N-(3-biphenyl-4-ylpropanoyl)-L-alpha-glutamyl-L-alpha-glutamyl-amide | C25 H29 N3 O7 | 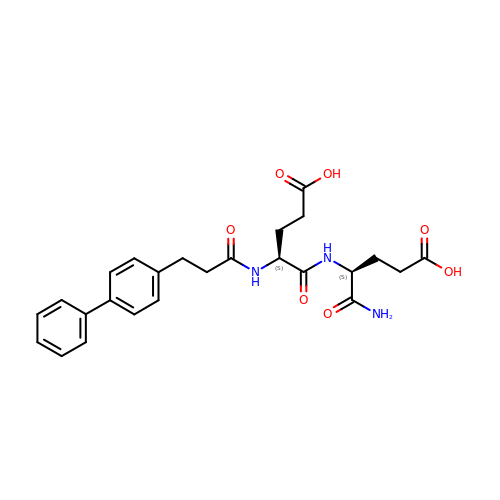KGICPKKIUBLFER-PMACEKPBSA-N> MSELEKAMVALIDVFHQYSGREGDKHKLKKSELKELINNELSHFLEEIKEQEVVDKVMETLDNDGDGECDFQEFMAFVAMVTTACH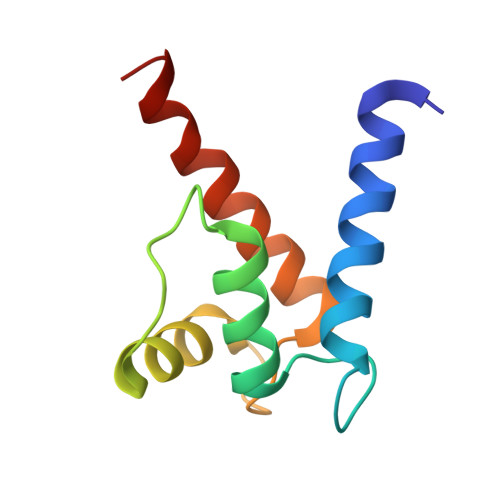EFFEHE>MAHHHHHHMVAMQSTIPSLTREEIADRMQHNPLVQAYQQEV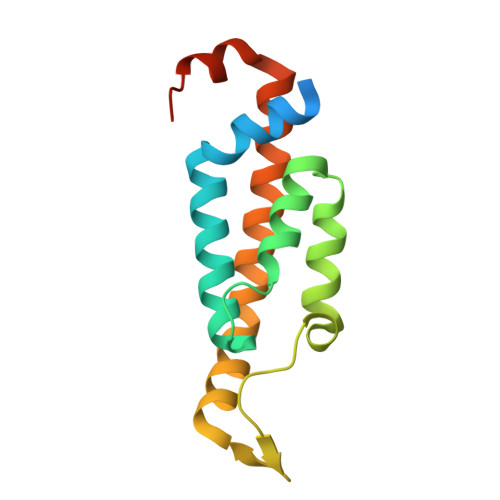MHWCKIVYGNSDVLKEKMQEVLQKPSEGEDLSRQVAENPTSVHKLAGRNLCGLKTNARRQAEEGFMHLCQALDGYTSAVTQAQENIKHVPQAEARRYGQESEQRA[4x]> MTMDEQQSQAVAPVYVGGFLARYDQSPDEAELLLPRDVVEHWLHAQGQGQPSLSVALPLNINHDDTAVVGHVAAMQSVRDGLFCLGCVTSPRFLEIVRRASEKSELVSRGPVSPLQPDKVVEFLSGSYAGLSLSSRRCDDVEQATSLSGSETTPFKHVALCSVGRRRGTLAVYGRDPEWVTQRFPDLTAADRDGLRAQWQR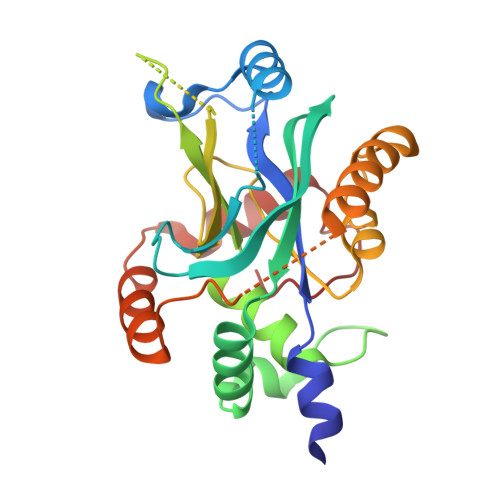CGSTAVDASGDPFRSDSYGLLGNSVDALYIRERLPKLRYDKQLVGVTERESYVKA>[2x]MGHHHHHHHHLVP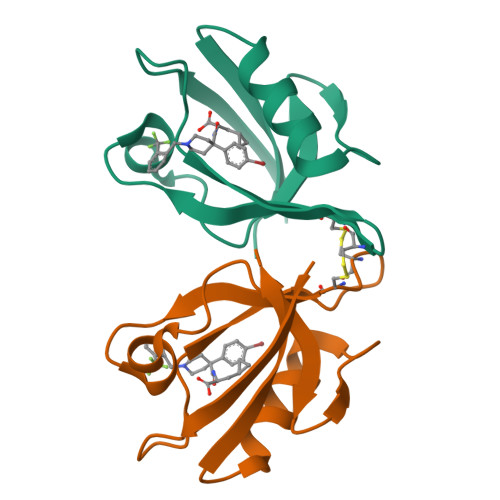RGSMFADLDYDIEEDKLGIPTVPGKVTLQKDAQNLIGISIGGGAQYCPCLYIVQVFDNTPAALDGTVAAGDEITGVNGRSIKGKTKVEVAKMIQEVKGEVTIHYNKLQQSAV> KCQLRFASLGDWGKDTKGQILNAKYFKQFIKNERVTFIVSPGSNFIDGVKGLNDPAWKNLYEDVYSEEKGDMYMPFFTVLGTRDWTGNYNAQLLKGQGIYIEKNGETSIEKDADATNYPKWIMPNYWYHYFTHFTVSSGPSIVKTGHKDLAAAFIFIDTWVLSSNFPYKKIHEKAWNDLKSQLSVAKKIADFIIVVGDQPIYSSGYSRGSSYLAYYLLPLLKDAEVDLYISGHDNNM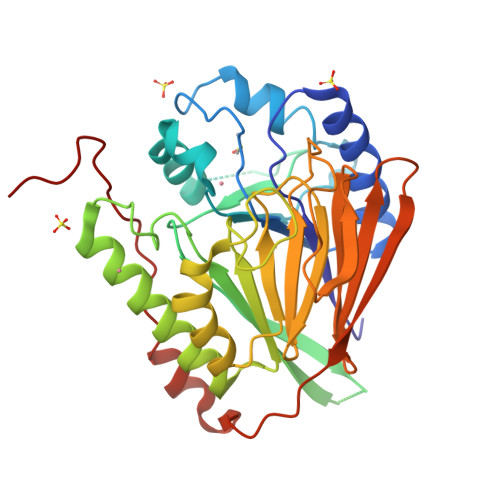EVIEDNDMAHITCGSGSMSQGKSGMKNSKSLFFSSDIGFCVHELSNNGIVTKFVSSKKGEVIYTHKLNIKKKKTLDKVNALQHFAALPNVELTDVPSSGPMGNKD> MVPISPIETVPVKLKPGMDGPKVKQWPLTEEKIKALVEICTEMEKEGKISKIGPENPYNTPVFAIKKKDSTKWRKLVDFRELNKRTQDFWEVQLGIPHPAGLKQKKSVTVLDVGDAFYSVPLDKDFRKYTAFTIPSINNETPGIRYQYNVLPMGWKG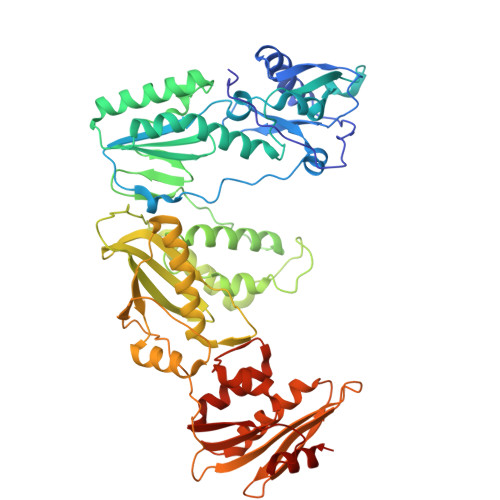SPAIFQSSMTKILEPFRKQNPDIVIYQYMDDLYVGSDLEIGQHRTKIEELRQHLLRWGFTTPDKKHQKEPPFLWMGYELHPDKWTVQPIVLPEKDSWTVNDIQKLVGKLNWASQIYAGIKVRQLSKLLRGTKALTEVVPLTEEAELELAENREILKEPVHGVYYDPSKDLIAEIQKQGQGQWTYQIYQEPFKNLKTGKYARMKGAHTNDVKQLTEAVQKIATESIVIWGKTPKFKLPIQKETWEAWWTEYWQATWIPEWEFVNTPPLVKLWYQLEKEPIIGAETFYVDGAANRETKLGKAGYVTDRGRQKVVPLTDTTNQKTELQAIHLALQDSGLEVNIVTDSQYALGIIQAQPDKSESELVSQIIEQLIKKEKVYLAWVPAHKGIGGNEQVDKLVSAG> MGLNFFRKAAPEVRTEPVAERKASVTGRIVAMASGAGRPVWGPRDTVSLMRTGFAGNPVGFRSVKLIAEATAAVPLICQDAERRYEIHPVLDLLRRPNAGQGRAELFEALIGQILLSGNGYLEAVCPEPGVPRELHVLRSDRMAVVPGADGWPVGYDYTVGG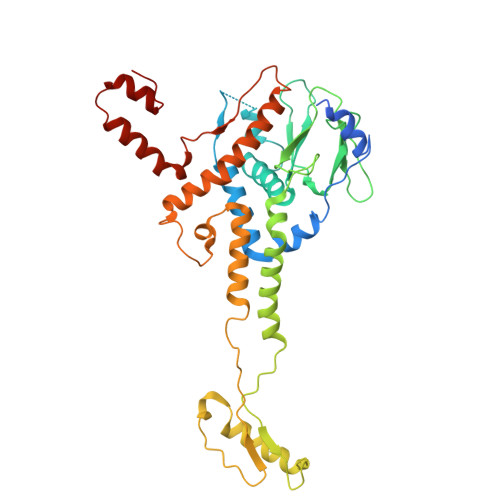RKHRFDMTGHPDPICHIKSFHPTDDHYGLSPMQAAAVALDVHNAASAWSKALLDNAARPSGAIIYKGADGQGVLAPEQYERLIFEMETHHQGARNAGRPMLLEGGLDWKPMGFSPSDMEFHETKAAAAREIALAFGVPPMLIGIPGDATYANYAEANRAFYRLTVLPLLTRVSAALAWWLSGYLGAQIELKPDLDQVPALAVERDQLWARIGAAGFLSNSEKRVLLGLPPT> SVAILQKRDHEGFGFVLRGAKAETPIEEFTPTPAFPALQYLESVDVEGVAWKAGL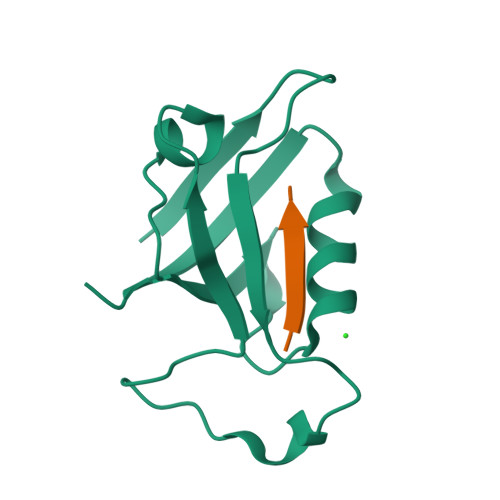RTGDFLIEVNGVNVVKVGHKQVVGLIRQGGNRLVMKVVSVT;> XEAQTRL Filamentous inoviruses such as MDAΦ are a genus of bacteriophages consisting of a single-stranded DNA (ssDNA) genome that is surrounded by an α-helical capsid, resulting in rod-like phage particles up to several micrometers in length but less than ten nanometers in diameter. In N. meningitidis, MDAΦ particles, after being secreted into the extracellular milieu, assemble into filament bundles that promote cohesion between cells, thus promoting the formation of biofilms. Here, we present the electron cryomicroscopy (cryo-EM) structure of native MDA inoviral bacteriophages isolated from N. meningitidis, revealing significant differences to previously solved inovirus capsid structures. Our structural data on the biomedically relevant MDA phage show that MDAΦ is a class I, C5-symmetric bacteriophage with dense MCP packing.

We estimated the helical parameters from two-dimensional class averages and employed real-space helical refinement to solve the structure of the MDAΦ MCP to 3.7 Å resolution. The resulting cryo-EM map reveals α-helical MCPs packed into a tubular arrangement, with an overall diameter of ~62 Å and a central pore with a ~20 Å diameter. MCPs are arranged with a pentameric (C5) rotational symmetry around the filament axis, with a rise of 14.1 Å and 42.3° rotation per subunit, establishing MDAΦ as a class I inovirus. Each MCP of MDAΦ adopts a bent architecture with significantly higher curvature than what has been seen in previous inovirus capsid structures, showing an angle of ~45° between the N- and the C-terminal segments of the MCP. The first six residues of the MCP are poorly resolved with smeared density in the cryo-EM map, suggesting flexibility of this region. Consistent with past structural data on inoviruses, the MCP of MDAΦ contains numerous hydrophobic residues in the central segment, which form an extensive hydrophobic network through tight packing with other MCP subunits around the filament axis. The helical parameters of the MDAΦ capsid (rise: 14.1 Å, right-handed rotation 42.3°) are markedly different from other C5-symmetric class I phages such as the Ff group of phages (fd phage rise 16.6 Å, fd phage rotation 36.4° to 37.5°) and IKe (rise 16.8 Å, rotation 38.5°), with a lower rise resulting in a comparably higher number of MCP proteins in any given capsid segment. The C-terminus of the MDAΦ MCP, which is exposed to the phage lumen, contains three lysine residues with side chains extending toward the phage genome. To ascertain how bundling is mediated at the molecular level, we inspected our atomic model of the MDAΦ MCP and noticed that the N-terminal residues 1–6 form a surface-exposed segment with a prominent hydrophobic phenylalanine residue (F3) in the poorly resolved, flexible N-terminus of the protein, which is followed by further hydrophobic residues 5–9 (sequence AAAI).

> DGFDAAAIGTQVANVIMGFVAMVSAVGMAAITVILAIQGFKMAWSMIKSVK>[6x]LEMRIGHGFDVHAFGGEGPIIIG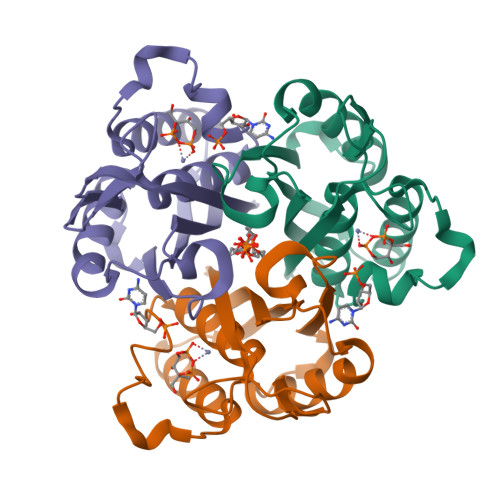GVRIPYEKGLLAHSDGDVALHALTDALLGAAALGDIGKLFPDTDPAFKGADSRELLREAWRRIQAKGYTLGNVDVTIIAQAPKMLPHIPQMRVFIAEDLGCHMDDVNVKATTTEKLGFTGRGEGIACEAVALLIKATK> 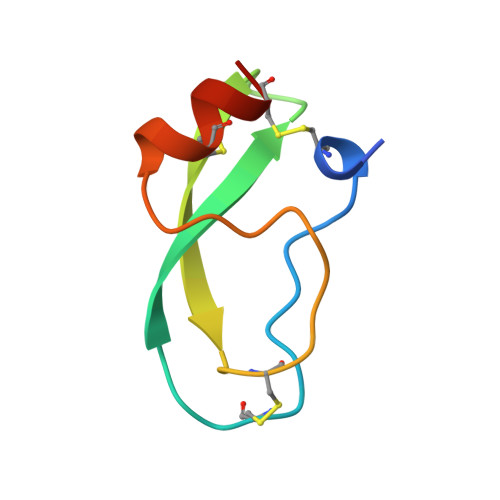VREVCSEQAETGPCRAMISRWYFDVTEGKCAPFFYGGCGGNRNNFDTEEYCMAVCGSA> GSHMELTEDLNMELRVFFDTNKSNIKDQYKPEIAKVAEKLSEYPN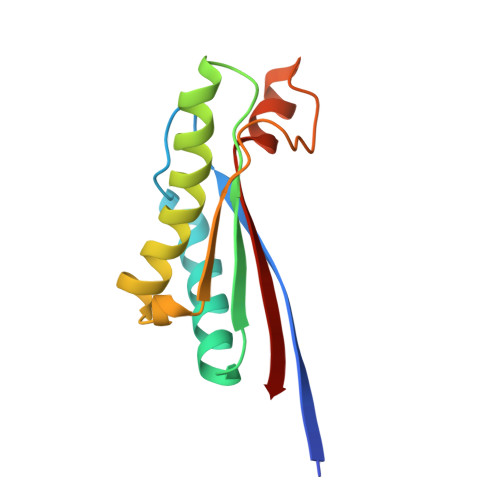ATARIEGHTDNTGPRKLNERLSLARANSVKSALVNEYNVDASRLSTQGFAWDQPIADNKTKEGRAMNRRVFATITGSR4-[4-[2-(1~{H}-indol-3-yl)ethyl]pyrimidin-2-yl]morpholine 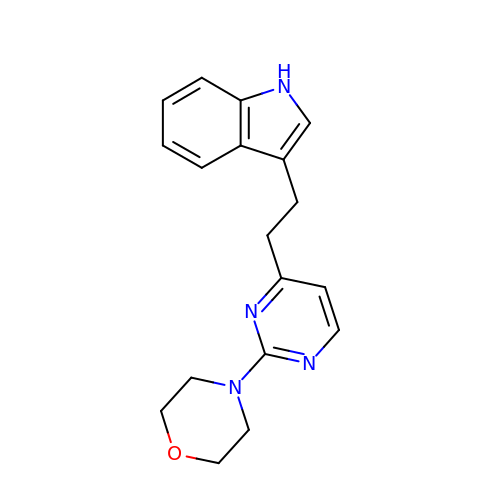| C18 H20 N4 O | UEMXDZGQUZIRAH-UHFFFAOYSA-N> MIIDSKTTLPRHSLIHTIKLNSNKKYGPGDMTNGNQFIISKQEWATIGAYIQTGLGLPVNEQQLRTHVNLSQDISIPSDFSQLYDVYCSDKTSAEWWNKNLYPLIIKSANDIASYGFKVAGDPSIKKDGYFKKLQDELDNIVDNNSDDDAIAKAIKDFKARCGILIKEAKQYEEAAKNIVTSLDQFLHGDQKKLEGVINIQKRLKEVQTALNQAHGESSPAHKELLEKVKNLKTTLERTIKAEQDLEKKVEYSFLLGPLLGFVVYEILENTAVQHIKNQIDEIKKQLDSAQHDLDRDVKIIGMLNSINTDIDNLYSQGQEAIKVFQKLQGIWATIGAQIENLRTTSLQEVQDSDDADEIQIELEDASDAWLVVAQEARDFTLNAYSTNSRQNLPINVISDSCNCSTTNMTSNQYSNPTTNMTSNQYMISHEYTSLPNNFMLSRNSNLEYKCPENNFMIYWYNNSDWYNNSDWYNN

The Cry6 family of proteins from Bacillus thuringiensis represents a group of powerful toxins with great potential for use in the control of coleopteran insects and of nematode parasites of importance to agriculture. One such Cry protein is Cry6Aa, a protein with activity against Coleoptera such as the Western Corn Rootworm Diabrotica virgifera virgifera and a range of nematodes, including both free-living (Caenorhabditis elegans and Panagrellus redivivus) and plant pathogenic (Heterodera glycines and Meloidogyne incognita) species that cause large-scale losses to agriculture. To increase our understanding of their mode of action and to facilitate further development of these proteins we have determined the structure of Cry6Aa in protoxin and trypsin-activated forms and demonstrated a pore-forming mechanism of action. The structures obtained are novel among invertebrate-active toxins and are consistent with Cry6Aa acting as a pore-forming toxin.

The structure of the trypsin-resistant core exhibits a group of long alpha helices (around 90 Å) that are amphipathic in nature, with their hydrophobic sides interacting and their hydrophilic faces showing greater exposure to solvent. This helix bundle is around 20–25 Å in diameter with a head domain folded across the helices at one end, formed from residues close to the C-terminus of the protein. Analysis of the trypsin-resistant core by SDS-PAGE following reduction and Edman degradation of the major band showed the N-terminal sequence HSLIH, corresponding to residues 12–16 of the Cry6Aa sequence and indicating processing after Arg11. The deconvoluted intact average molecular weight (MWavg) value of 46,844.19 Da matches the theoretical value (46,843.43 Da) expected for a core protein containing polypeptide chain 12–390 disulfide bonded to chain 444–475 with a mass error of +16.2 ppm. The 3266.38 peak had the sequence CPENNFMIYWYNNSDWYNNSDWYNN, which matched the CTP2 sequence from residues 451–475. These results show trypsin cleavage after Arg390 and processing sites after Arg443 and, at a lower frequency, after Lys450. The solved structure of the trypsin-activated Cry6Aa corresponds to the major core of the toxin with the longer CTP1 fragment (from Asn444 to Trp472) still linked to the main body of the toxin by a disulfide bond. This bond can be clearly resolved in the structure (insert). However, several residues were not resolved in the activated toxin structure: CTP1 residues Asn444 and Tyr473-Asn475; core region residues Lys126-Lys127 and Asn388-Ser389-Arg390, indicating that these regions are not fixed in the structure.> MSYPEKFEGIAIQSHEDWKNPKKTKYDPKPFYDHDIDIKIEACGVCGSDIHCAAGHWGNMKMPLVVGHEIVGKVVKLGPKSNSGLKVGQRVGVGAQVFSCLECDRCKN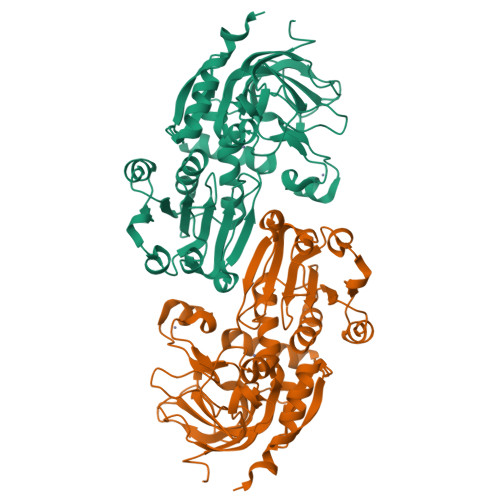DNEPYCTKFVTTYSQPYEDGYVSQGGYANYVRVHEHFVVPIPENIPSHLAAPLLCGGLTVYSPLVRNGCGPGKKVGIVGLGGIGSMGTLISKAMGAETYVISRSSRKREDAMKMGADHYIATLEEGDWGEKYFDTFDLIVVCASSLTDIDFNIMPKAMKVGGRIVSISIPEQHEMLSLKPYGLKAVSISYSALGSIKELNQLLKLVSEKDIKIWVETLPVGEAGVHEAFERMEKGDVRYRFTLVGYDKEFSD> MAESKPTPQSTFTGPIVVDPITRIEGHLRIMVEVENGKVKDAWSSSQLFRGLEIILKGRDPRDAQHFTQRACGVCTYVHALASSRCVDDAVKVSIPANARMMRNLVMASQYLHDHLVHFYHLHALDWVDVTAALKADPNKAAKLAASIAPARPGNSAKALKAVQDKLKAFVESGQLGIFTNAYFLGGHKAYYLPPEVNLIATAHYLEALHMQVKAASAMAILGGKNPHTQFTVVGGCSNYQGLTKDPLANYLALSKEVCQFVNECYIPDLLAVAGFYKDWGGIGGTSNYLAFGEFATDDSSPSKHLATSQFPSGVITGRDLGKVDNVDLGAIYEDVKYSWYAPGGDGKHPYDGVTDPKYTKLDDKDHYSWMKA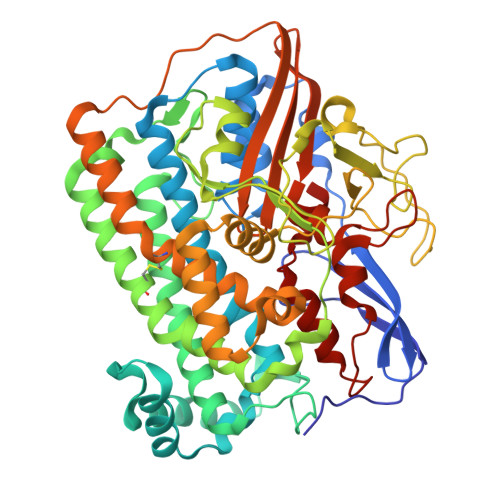PRYKGKAMEVGPLARTFIAYAKGQPDFKKVVDMVLGKLSVPATALHSTLGRTAARGIETAIVCANMEKWIKEMADSGAKDNTLCAKWEMPEESKGVGLADAPRGALSHWIRIKGKKIDNFQLVVPSTWNLGPRGAQGDKSPVEEALIGTPIADPKRPVEILRTVHAFDPCIACGVH> SMGRGSGTFERLLDKATSQL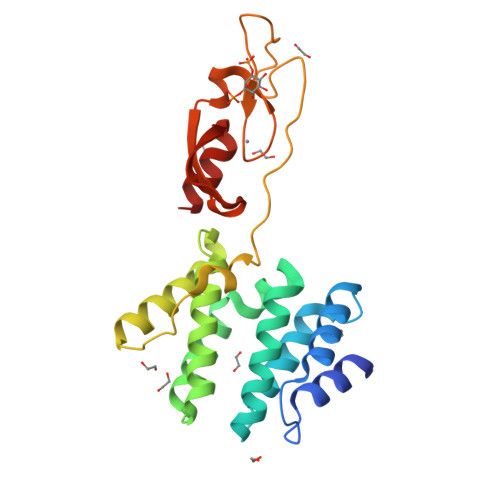LLETDWESILQICDLIRQGDTQAKYAVNSIKKKVNDKNPHVALYALEVMESVVKNCGQTVHDEVANKQTMEELKDLLKRQVEVNVRNKILYLIQAWAHAFRNEPKYKVVQDTYQIMKVEGHVFPEFKESDAMFAAERAPDWVDAEECHRCRVQFGVMTRKHHCRACGQIFCGKCSSKYSTIPKFGIEKEVRVCEPCYEQLNRKAEG> MFARLIRYFQEARAELARVTWPTREQVVEGTQAILLFTLAFMVILGLYDTVFRFLIGLLR;> MDLLYTLVILFYLGVAGLLVYLVLVQEPKQGAGDLMGGSADLFSARGVTGGLYRLTVILGVVFAALALVIGLWPR;> MVKAFWSALQIPELRQRVLFTLLVLAAYRLGAFIPTPGVDLDKIQEFLRTAQGGVFGIINLFSGGNFERFSIFALGIMPYITAAIIMQILVTVVPALEKLSKEGEEGRRIINQYTRIGGIALGAFQGFFLATAFLGAEGGRFLLPGWSPGPFFWFVVVVTQVAGIALLLWMAERITEYGIGNGTSLIIFAGIVVEWLPQILRTIGLIRTGEVNLVAFLFFLAFIVLAFAGMAAVQQAERRIPVQYARGAAGYGGQATYIPIKLNAAGVIPIIFAAAILQIPIFLAAPFQDNPVLQGIANFFNPTRPSGLFIEVLLVILFTYVYTAVQFDPKRIAES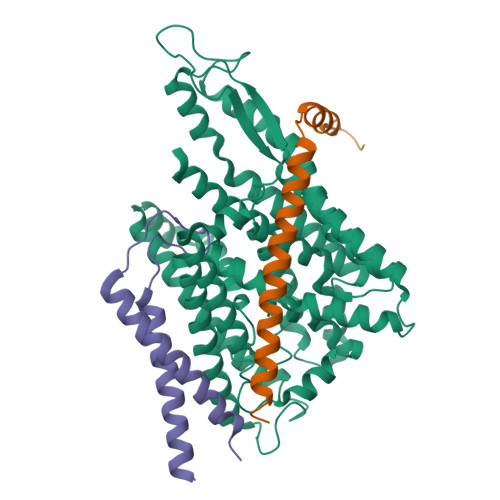LREYGGFIPGIRPGEPTVKFLEHIVSRLTLWGALFLGLVTLLPQIIQNLTGIHSIAFSGIGLLIVVGVALDTLRQVESQLMLRSYEGFLSRGRLRGRNRHHHHHH>[6x]MEAIRKELSRSYQELNEEAEPVAIDPEEAEDEEKEQEEAASAVAPDRDSDRSSPPVRF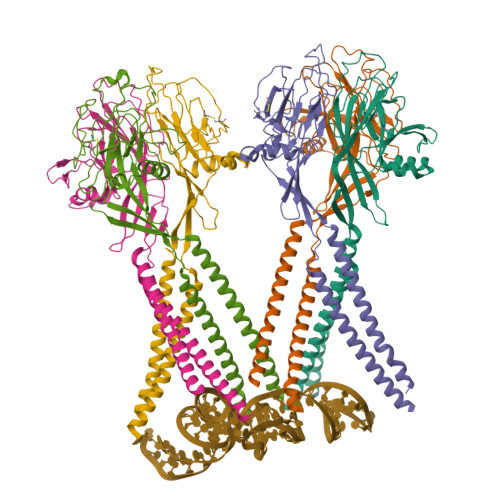SRTCLKNFFSVLLILVYLLLMGVAVFLVYQTITDFRDKLKHPVMSVSYKEVNMYDAPGIALYPGKARLLSCEHHWYDHIPPLKDPGQPGENTCVTQDISYIDPYTNKTMKHALIVQGPRDVRRRELVFLQFHLNETKQDFSAIDYLLFSSYEAFLKSHDQVKFMQDCESSFSSWKFSGGFRTWVKMSLVKTKEEDGSQSVEFRQETSVVNFIDRRETPDKGDQLFFVVFEWKDPYIQEIQDIITANPWSMIALLCSVFLVLFKAADFAKLSVKWMIKVRRRHLKKRARELNHIS>SNADAKKNPKSSKFPAPSEGLATAKANQGGIPKQVLSDASWTYGEGAALDTVAASAPVLDIYFDYSCSHCAQFEGLHTQEINQLLSDKKITLALHPCKLLQQEWTSVVMNAMGVVLDEAPAQSLSFHNAAFEIFSQAIQTKNQSNMTVEGLVAAAA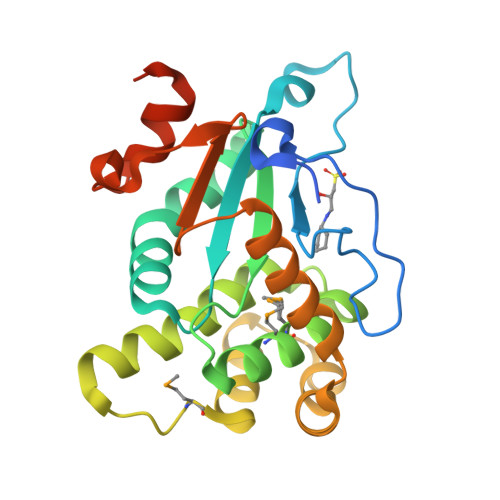KVNVPKEVSAKFKAAVDSDKYGKWVKLGDEAFKARELEGTPTVFFKGEKVDLNKLQTPTSLTELVTGSTPTAQPSPQPTQQG[2x]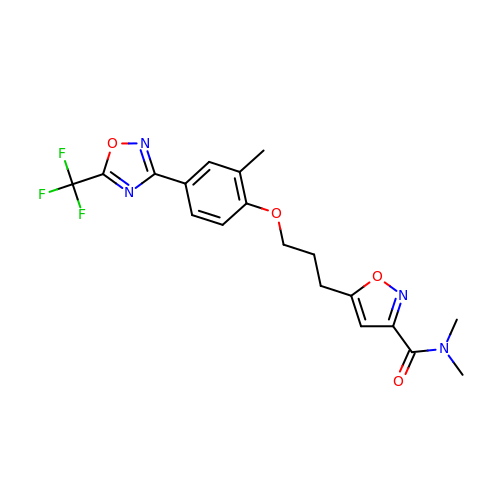N,N-dimethyl-5-(3-{2-methyl-4-[5-(trifluoromethyl)-1,2,4-oxadiazol-3-yl]phenoxy}propyl)-1,2-oxazole-3-carboxamide | C19 H19 F3 N4 O4 | ZDMWUMVBMYLHFC-UHFFFAOYSA-N> SNASYRSTQQITDFTKEILVNGEAVTAFDRQGDLPNVVVTPNFEAGVDQVVDQLAMNDSERD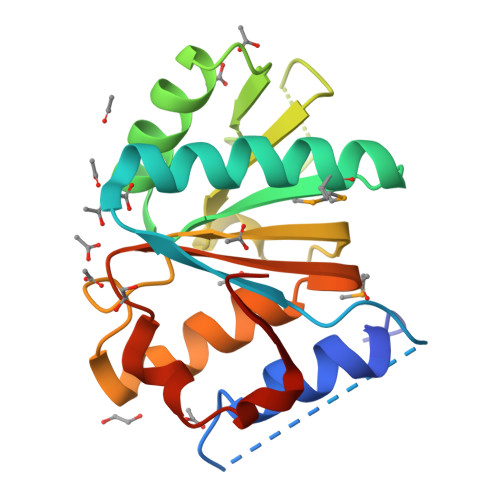TTAIIGKSLAECEALTKALKARGEQVTLIQTENQRLAPGVIVVPSFLAKGLEFDAVIVWNANQENYQREDERQLLYTICSRAMHELTLVAVGSLSPLLARVNHALYTLNEAK>MSEQYSEINTDTLERVTEIFKALGDYNRIRIMELLSVSEASVGHISHQLNLSQSNVSHQLKLLKSLHLVKAKRQ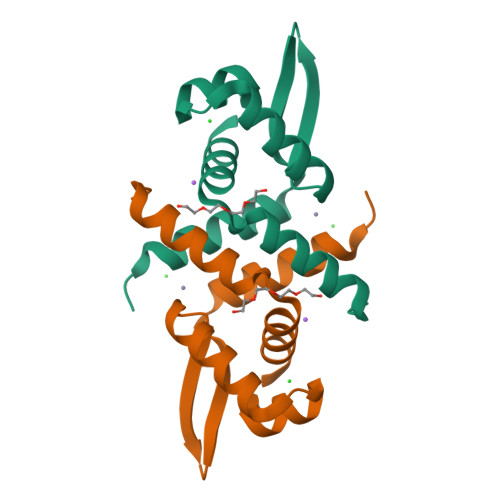GQSMIYSLDDIHVATMLKQAIHHANHPKESGL[2x]>[2x]GMLEGLEAVRKRPGMYIGSTGERGLHHLIWEVVDNAVDEAMAGHATKVRVRLLADGG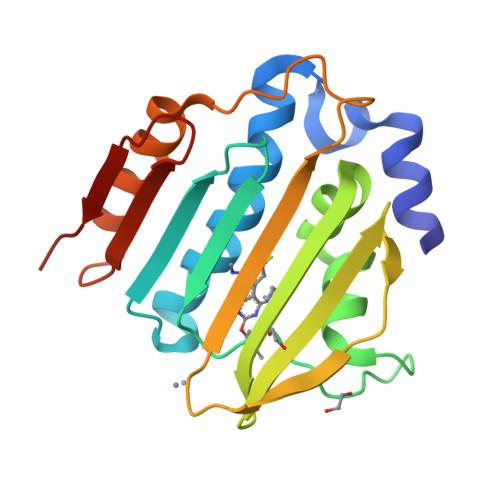VEVSDDGRGIPVEMHESGVPTVDVVMTQVGVSVVNALSTRMEVEICRDGYQWFQTYDKSVPGTLKQGEKTRKTGTVVRFWPDPDVFETTTFDFETVARRLQEQAFLNKGLTIELIDERDGKHRTFYYPG>[8x]MYFEIYKDAKGEYRWRLKAA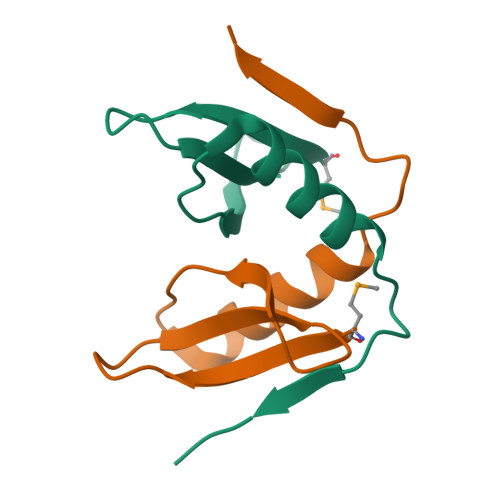NHEIIAQGEGYTSKQNCQHAVDLLKSTTAATPVKEVLEHHHHHH>MGSSHHHHHHSAALEVLFQGPDYKFWYTQPVPKINDEFNESVNEPFISDNKVEDVRKDEYKLPPGYSWYVCDVKDEKDRSEIYTLLTDNYVEDDDNIFRFNYSAEFLLWALTSPNYLKTWHIGVKYDASNKLIGFISAIPTDICIHKRTIKMAEVNFLCVHKTLRSKRLAPVLIKEITRRINLENIWQAIYTAGVYLPKPVSDARYYHRSINVKKLIEIGFSSLNSRLTMSRAIKLYRVEDTLNIKNMRLMKKKDVEGVHKLLGSYLEQFNLYAVFTKEEIAHWFLPIENVIYTYVNEENGKIKDMISFYSLPSQILGNDKYSTLNAAYSFYNVTTTATFKQLMQDAILL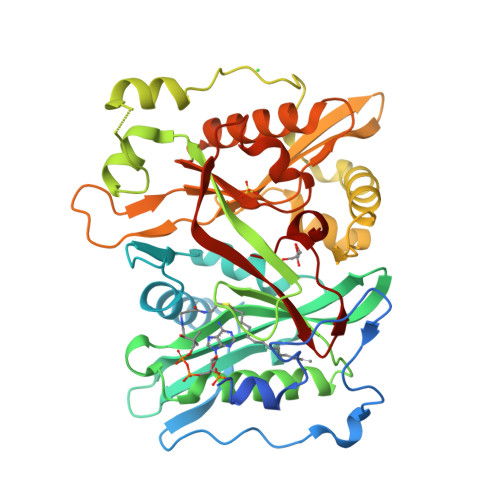AKRNNFDVFNALEVMQNKSVFEDLKFGEGDESLKYYLYNWKCASFAPAHVGIVLL[3x]> GPGSTTYIFGKGGALITYTWPPNDRPSTRMDRLAVGFSTHQRSAVLVRVDSASGLGDYLQLHIDQGTVGVIFNVGTDDITIDEPNAIVSDGKYHVVRFTRSGGNATLQVDSWPVNERYPAGNFDNERLAIARQRIPYRLG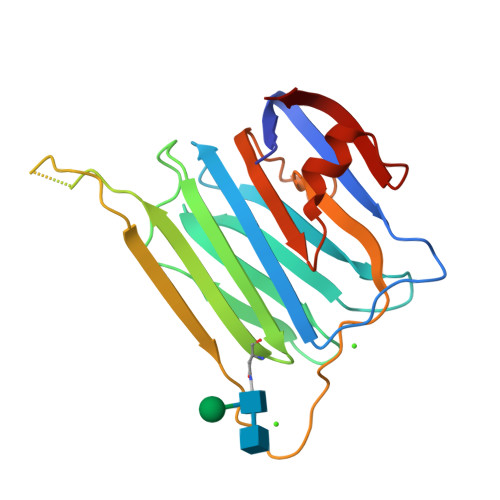RVVDEWLLDKGRQLTIFNSQATIKIGGRDQGRPFQGQVSGLYYNGLKVLALAAESDPNVRTEGHLRLV> SDTERPVVNVPSEITVYRGESFEYFATVTDNSNAFDLAKTVVRWLYSNQPGRGTEWLQYSVTQVGNQLKVRIFGNVPIDTTIGDYTRYVVATDAAGNVNATQTEMGNAAVDKTS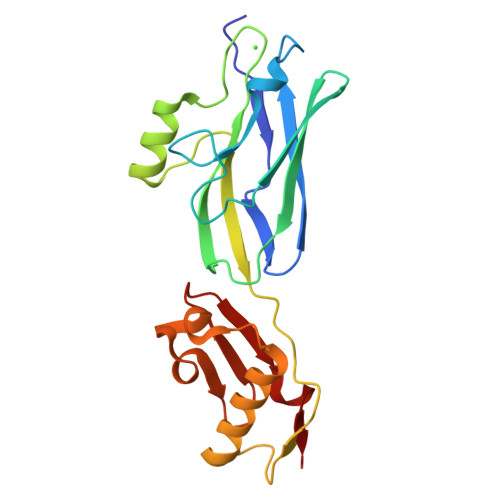VNGQFKLIIRFRIKTPENTVFVNNPNQLTEVEKNLVREAVKKSNPDLRAQDVLNSNYVTGITVSNNGTTTITYRDGRKDIIDGSKFIDTR A broad and rich body of literature based on decades of study describes the biochemical and functional properties of KATP channels (Aguilar-Bryan and Bryan, 1999; Aguilar-Bryan et al., 1998; Ashcroft et al., 2017; Ashcroft and Ashcroft, 1992; Hibino et al., 2010; Nichols, 2016; 2006). These channels were found to be large oligomeric complexes composed of four sulphonylurea receptor (SUR) subunits, which belong to the ABCC family of ABC transporters, and four Kir6 subunits, which are members of the inward rectifier potassium channel family. The focus of this study is the human KATP channel composed of SUR1 and Kir6.2, which are found in pancreatic beta cells where they play a major role in regulating insulin secretion. By virtue of their sensitivity to both ATP and ADP, these channels are thought to couple cellular metabolism to membrane excitability. Three naturally occurring ligands control the activity of KATP channels: PIP2 is required for activity, ATP inhibits activity, and ADP potentiates activity.

In the quatrefoil form, KATP is a symmetrical tetramer; each protomer consists of one K+ channel subunit and one ABC transporter. The TMD0s are bound to the channel and hold the four ABC transporters akin to the leaves of a quatrefoil. Upon further classification and refinement, the propeller form was determined to 5.6 Å resolution and the quatrefoil form was determined to 3.9 Å resolution. EM density of the entire complex is very well defined, but residues 193–261, known as the L0-loop, containing a conserved lasso motif is not visible. Mg2+-ATP is bound in the ‘closed’ catalytically inactive degenerate site and Mg2+-ADP is bound in the ‘open’ catalytically competent consensus ATPase site. In this structure, both the inner helix gate and the G-loop gates are closed. Four ATP molecules are associated with the Kir6.2 channel (one ATP per subunit); each binds in a shallow pocket on the surface of the CTD. Formation of the quatrefoil form is associated with disruption of the lasso extension/ATP-binding site interface. In the quatrefoil form, the SUR1 transport modules reside coplanar, that is, in the same hydrophobic plane as defined by the Kir6 and TMD0 elements. In the quatrefoil form, we observe a new interface formed between SUR1 and the Kir6.2 CTD near the ADP-binding site.

>[4x]SASASAMLSRKGIIPEEYVLTRLAEDPAEPRYRARQRRARFVSKKGNCNVAHKNIREQGRFLQDVFTTLVDLKWPHTLLIFTMSFLCSWLLFAMAWWLIAFAHGDLAPSEGTAEPCVTSIHSFSSAFLFSIEVQVTIGFGGRMVTEECPLAILILIVQNIVGLMINAIMLGCIFMKTAQAHRRAETLIFSKHAVIALRHGRLCFMLRVGDLRKSMIISATIHMQVVRKTTSPEGEVVPLHQVDIPMENGVGGNSIFLVAPLIIYHVIDANSPLYDLAPSDLHHHQDLEIIVILEGVVETTGITTQARTSYLADEILWGQRFVPIVAEEDGRYSVDYSKFGNTIKVPTPLCTARQLDEDHSLLEALTLASARGPLRKRSVPMAKAKPKFSISPDSLSSNSLEVLFQG;>[4x]MPLAFCGSENHSAAYRVDQGVLNNGCFVDALNVVPHVFLLFITFPILFIGWGSQSSKVHIHHSTWLHFPGHNLRWILTFMLLFVLVCEIAEGILSDGVTESHHLHLYMPAGMAFMAAVTSVVYYHNIETSNFPKLLIALLVYWTLAFITKTIKFVKFLDHAIGFSQLRFCLTGLLVILYGMLLLVEVNVIRVRRYIFFKTPREVKPPEDLQDLGVRFLQPFVNLLSKGTYWWMNAFIKTAHKKPIDLRAIGKLPIAMRALTNYQRLCEAFDAQVRKDIQGTQGARAIWQALSHAFGRRLVLSSTFRILADLLGFAGPLCIFGIVDHLGKENDVFQPKTQFLGVYFVSSQEFLANAYVLAVLLFLALLLQRTFLQASYYVAIETGINLRGAIQTKIYNKIMHLSTSNLSMGEMTAGQICNLVAIDTNQLMWFFFLCPNLWAMPVQIIVGVILLYYILGVSALIGAAVIILLAPVQYFVATKLSQAQRSTLEYSNERLKQTNEMLRGIKLLKLYAWENIFRTRVETTRRKEMTSLRAFAIYTSISIFMNTAIPIAAVLITFVGHVSFFKEADFSPSVAFASLSLFHILVTPLFLLSSVVRSTVKALVSVQKLSEFLSSAEIREEQCAPHEPTPQGPASKYQAVPLRVVNRKRPAREDCRGLTGPLQSLVPSADGDADNCCVQIMGGYFTWTPDGIPTLSNITIRIPRGQLTMIVGQVGCGKSSLLLAALGEMQKVSGAVFWSSLPDSEIGEDPSPERETATDLDIRKRGPVAYASQKPWLLNATVEENIIFESPFNKQRYKMVIEACSLQPDIDILPHGDQTQIGERGINLSGGQRQRISVARALYQHANVVFLDDPFSALDIHLSDHLMQAGILELLRDDKRTVVLVTHKLQYLPHADWIIAMKDGTIQREGTLKDFQRSECQLFEHWKTLMNRQDQELEKETVTERKATEPPQGLSRAMSSRDGLLQDEEEEEEEAAESEEDDNLSSMLHQRAEIPWRACAKYLSSAGILLLSLLVFSQLLKHMVLVAIDYWLAKWTDSALTLTPAARNCSLSQECTLDQTVYAMVFTVLCSLGIVLCLVTSVTVEWTGLKVAKRLHRSLLNRIILAPMRFFETTPLGSILNRFSSDCNTIDQHIPSTLECLSRSTLLCVSALAVISYVTPVFLVALLPLAIVCYFIQKYFRVASRDLQQLDDTTQLPLLSHFAETVEGLTTIRAFRYEARFQQKLLEYTDSNNIASLFLTAANRWLEVRMEYIGACVVLIAAVTSISNSLHRELSAGLVGLGLTYALMVSNYLNWMVRNLADMELQLGAVKRIHGLLKTEAESYEGLLAPSLIPKNWPDQGKIQIQNLSVRYDSSLKPVLKHVNALIAPGQKIGICGRTGSGKSSFSLAFFRMVDTFEGHIIIDGIDIAKLPLHTLRSRLSIILQDPVLFSGTIRFNLDPERKCSDSTLWEALEIAQLKLVVKALPGGLDAIITEGGENFSQGQRQLFCLARAFVRKTSIFIMDEATASIDMATENILQKVVMTAFADRTVVTIAHRVHTILSADLVIVLKRGAILEFDKPEKLLSRKDSVFASFVRADK> GHMNAADRVMQSYGRCCASTGFFDDFYRHFLASSPQIRAKFATTDMTAQKHLLRAGIMNLVMYARGMSDSKLRALGASHSRAALDIRPELYDLWLDALLMAVAEHDRDCDAETRDAWRDVMGRGIAV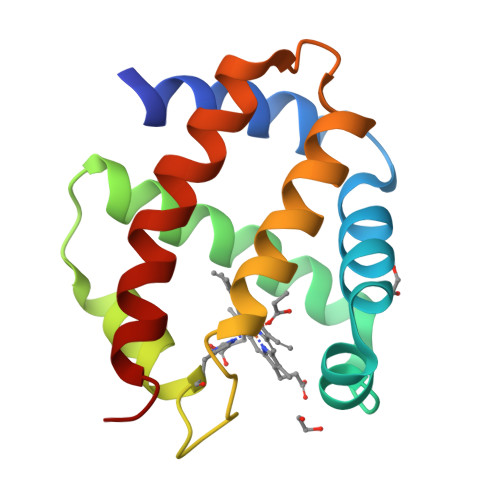IKSYYGS> GSMDALNFVTAIRGLINEQVAEVHTSLPVRVIGVDYGSKTVTLESIVKNTRSTEDEIDYPTFHDVPFMVNGGGTGRI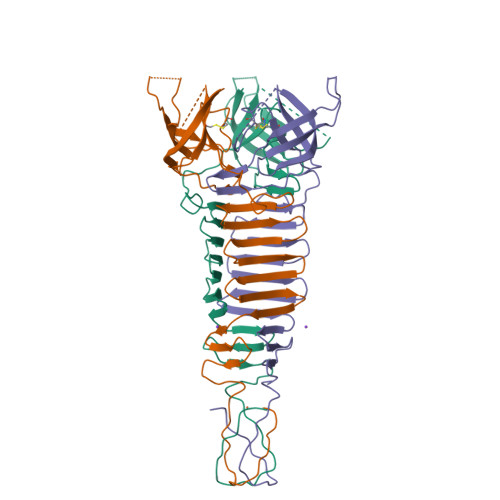SFPIKAGDIGVVVFSERDPSNAFQTDGDTASSGTLIQPCGLYPACFIPKIATATDSSEEVDSEKVIISNNKQTYASFDPNGNISVYNTQGMKIDMTPNSIVLTDAGGGKLTLQGGTMTYKGGTVNLNGLTITPDGRMTDSGGIGLHTHTHPVRGVETGGSTVTSDKPNGG>[4x]AQLVDSMPSASTGSVVVTDDLNYWGGRRIKSKDGATTEPVFEPATGRVLCQMVPCGAEEVDQAVQSAQAAYLKWSKMAGIERSRVMLEAARIIRERRDNIAKLEVINNGKTITEAEYDIDAAWQCIEYYAGLAPTLSGQHIQLPGGAFAYTRREPLGVCAGILAWNYPFMIAAWKCAPALACGNAVVFKPSPMTPVTGVILAEIFHEAGVPVGLVNVV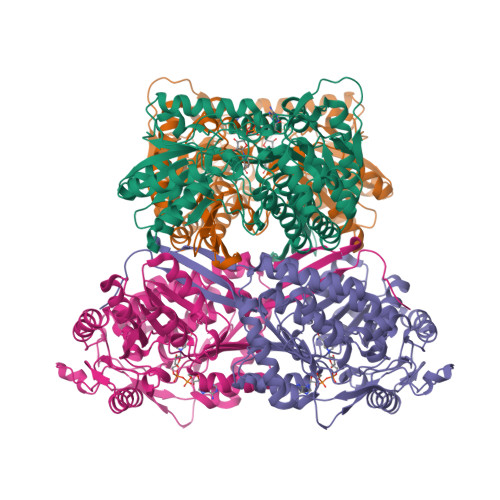QGGAETGSLLCHHPNVAKVSFTGSVPTGKKVMEMSAKTVKHVTLELGGKSPLLIFKDCELENAVRGALMANFLTQGQVCTNGTRVFVQREIMPQFLEEVVKRTKAIVVGDPLLTETRMGGLISKPQLDKVLGFVAQAKKEGARVLCGGEPLTPSDPKLKNGYFMSPCVLDNCRDDMTCVKEEIFGPVMSVLPFDTEEEVLQRANNTTFGLASGVFTRDISRAHRVAANLEAGTCYINTYSISPVEVPFGGYKMSGFGRENGQATVDYYSQLKTVIVEMGDVDSLF>[26x]MQKYALHAYPVMALMVATLTGCAWIPAKPLVQGATTAQPIPGPVPVANGSIFQSAQPINYGYQPLFEDRRPRNIGDTLTIVLQENVSASKSSSANASRDGKTSFGFDTVPRYLQGLFGNSRADMEASGGNSFNGKGGANASNTFSGTLTVTVDQVLANGNLHVVGEKQIAINQGTEFIRFSGVVNPRTISGSNSVPSTQVADARIEYVGNGYINEAQNMGWLQRFFLNLSPM;>MFKALAGIVLALVATLAHAERIRDLTSVQGVRENSLIGYGLVVGLDGTGDQTTQTPFTTQTLNNMLSQLGITVPTGTNMQLKNVAAVMVTASYPPFARQGQTIDVVVSSMGNAKSLRGGTLLMTPLKGVDSQVYALAQGNILVGGAGASAGGSSVQVNQLNGGRITNGAIIERELPTQF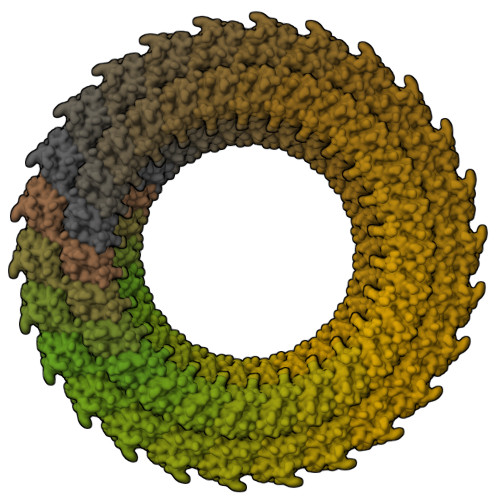GAGNTINLQLNDEDFTMAQQITDAINRARGYGSATALDARTVQVRVPSGNSSQVRFLADIQNMEVNVTPQDAKVVINSRTGSVVMNREVTLDSCAVAQGNLSVTVNRQLNVNQPNTPFGGGQTVVTPQTQIDLRQSGGSLQSVRSSANLNSVVRALNALGATPMDLMSILQSMQSAGCLRAKLEII[26x]> MEFVAKL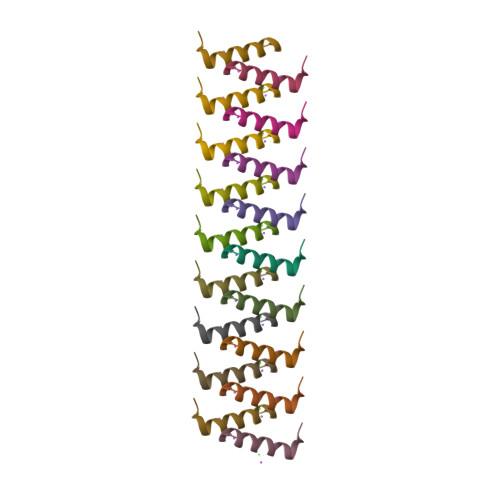FKFFKDLLAKFLGNN> GPGSEFELPLPEGWEEARDFDGKVYYIDHRNRTTSWIDPRDRYTKPLTFADCISDELPLGWEEAYDPQVGDYFIDHNTKTTQIEDPRVQWRREQEHMLKDYLVVAQEALSAQKEIYQVKQQRLELAQQEYQQLH;> GPGSRPKNMTPYRSPPPYVPP

WW domains organize molecular assemblies by binding to short, proline rich peptide motifs each with ~4–6 residues. The type I WW domains bind to a consensus ‘PPxY’ motif (where P is proline, x is any amino acid and Y is tyrosine, also known as PY-motif) with very modest affinities (with Kd in the range of a few to a few tens of µM). To achieve this goal, we determined the high resolustion structures of 7 representative WW tandem/target complexes, and measured the binding constants of >100 WW domain tandems or isolated WW domains binding to known or previously unknown targets. In this study, we discovered that WW tandems, but not individual WW domains, can bind to target proteins with extremely high affinity and with very high sequence specificity.

Taken all above results together, we can deduce a consensus sequence motif for specific and strong bindings to the WW-tandems of KIBRA, MAGI2, and MAGI3 as: ‘ΦΦxYxxΨPxY’, where Φ is aliphatic or small polar amino acids and Ψ can be Pro, Cys, Ala, Ser, Thr or Val. We searched for proteins in the UniProtKB/Swiss-Prot database and identified 132 human proteins containing the ‘ΦΦxYxxΨPxY’ motifs. We selected 7 of such consensus sequences from six proteins (JCAD, USP6NL, β-Dystroglycan, PTPN21, ABLIM-1, and PTCH1) to measure their bindings to the KIBRA and MAGI3 WW tandems by ITC. Interestingly, β-Dystroglycan, a protein known to play critical roles in Hippo signaling-related cell adhesion and cell growth (Morikawa et al., 2017; Gawor and Prószyński, 2018), can also bind to KIBRA WW tandem with a high affinity (Kd ~96 nM). We solved the crystal structure of the KIBRA WW tandem in complex with the β-Dystroglycan PY34 peptide. The complex structure confirmed that the peptide binds to the KIBRA WW tandem following the mode exactly as we have predicted. Therefore, β-Dystroglycan may be a key regulator in cell growth and neuronal synaptic functions via specifically binding to KIBRA.Enolase, a ubiquitous enzyme, catalyzes the reversible conversion of 2-phospho­glycerate (2PG) to phospho­enolpyruvate (PEP) in the glycolytic pathway of organisms of all three domains of life. Here we present structural snapshots of Mycobacterium tuberculosis (Mtb) enolase in apo, PEP-bound and two 2PG-bound forms as it catalyzes the conversion of PEP to 2PG. MtEno has a topology similar to other enolase structures, a smaller N-terminal domain and a larger C-terminal domain. The crystal and the cryoEM structures (enzyme in solution, frozen) along with the biochemical studies clearly demonstrate that the functional unit of MtEno is an octamer.

The octameric fraction was further used for structural studies. The structure of enolase in the apo state was determined using both cryoEM and X-ray crystallography. Freezing of apo–MtEno and PEP–MtEno at 3.5 mg ml−1 was accomplished with glow discharged Quantifoil holey carbon grids (R 0.6/1, Au 300 mesh) and a Vitrobot Mark IV set at 100% humidity and 16°C, with blotting for 3.5 s. Both the apo and the PEP–enolase data were collected in the Titan Krios at the National CryoEM facility, Bangalore, with a Falcon 3 detector in counting mode at 1.07 Å pixel−1 sampling with images exposed for 60 s, with a total accumulated dose of ∼27.70 e− Å−2 and dose fractionated into 25 frames, with each frame having a dose of ∼1.1 e− Å−2. Particles were extracted with a box size of 320 pixels and subjected to two rounds of 2D classification followed by 3D auto-refinement, per particle CTF refinement, B-factor weighting with Bayesian polishing and refinement, and subsequent 3D classification in RELION-3.0 with D4 symmetry imposed. The nominal resolutions of apo–MtEno and PEP–MtEno were 3.1 and 3.2 Å respectively.

>MHHHHHHMPIIEQVRAREILDSRGNPTVEVEVALIDGTFARAAVPSGASTGEHEAVELRDGGDRYGGKGVQKAVQAVLDEIGPAVIGLNADDQRLVDQALVDLDGTPDKSRLGGNAILGVSLAVAKAAADSAELPLFRYVGGPNAHILPVPMMNILNGGAHADTAVDIQEFMVAPIGAPSFVEALRWGAEVYHALKSVLKKEGLSTGLGDEGGFAPDVAGTTAALDLISRAIESAGLRPGADVALALDAAATEFFTDGTGYVFEGTTRTADQMTEFYAGLLGAYPLVSIEDPLSEDDWDGWAALTASIGDRVQIVGDDIFVTNPERLEEGIERGVANALLVKVNQIGTLTETLDAVTLAHHGGYRTMISHRSGETEDTMIADLAVAIGSGQIKTGAPARSERVAKYNQLLRIEEALGDAARYAGDLAFPRFACETK[8x]> MGHHHHHHLESTSLYKKSSSTPPRGVTVVNNFDCKRYLGTWYEIA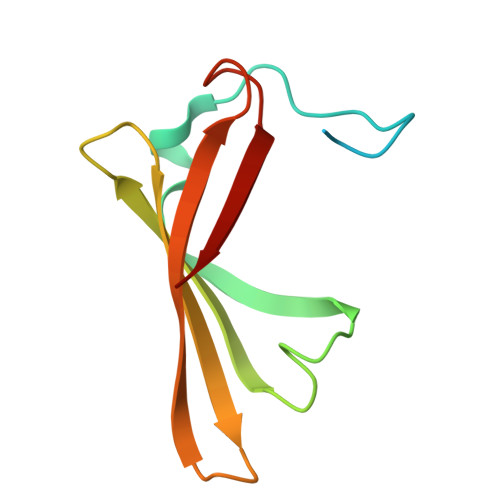RFDHRAERGLEKVTATYSLRDDGGLNVIFKGYNPDRGMWQQYVGKAYFTGAPTRAALKVAFF>MSQEIRQNEKISYRIEGPFFIIHLINPDNLNALEGEDYIYLGELLEL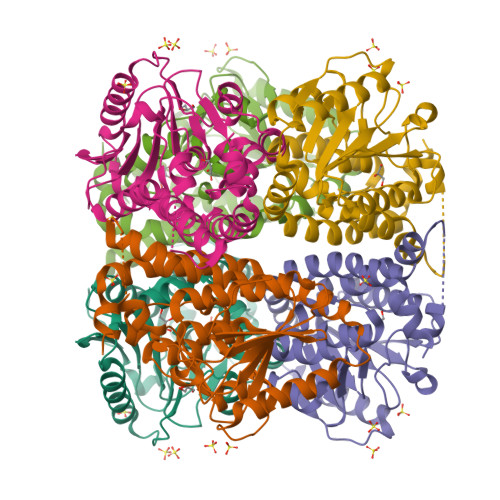ADRNRDVYFTIIQSSGRFFSSGADFKGIAKAQGDDTNKYPSETSKWVSNFVARNVYVTDAFIKHSKVLICCLNGPAIGLSAALVALCDIVYSINDKVYLLYPFANLGLITEGGTTVSLPLKFGTNTTYECLMFNKPFKYDIMCENGFISKNFNMPSSNAEAFNAKVLEELREKVKGLYLPSCLGMKKLLKSNHIDAFNKANSVEVNESLKYWVDGEPLKRFRQLGSKQRKHRL[3x]(1R,4S,5S,6R)-4-amino-5,6-dihydroxy-2-(hydroxymethyl)cyclohex-2-en-1-yl 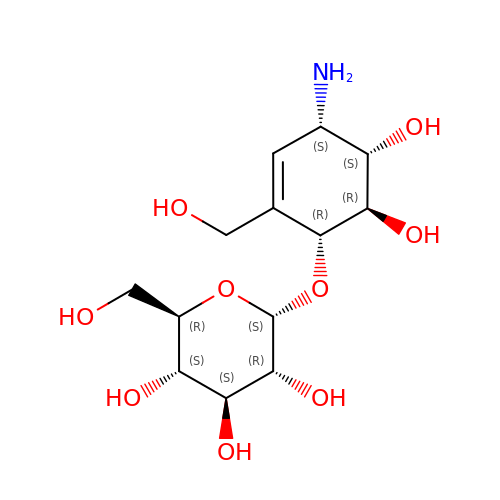alpha-D-glucopyranoside | C13 H23 N O9 | UINFOZNGFLXUEC-QHWKHWDXSA-N>[2x]GMRNELPPENAYRILESGPIVLVSTRGADGRANLMTMGFH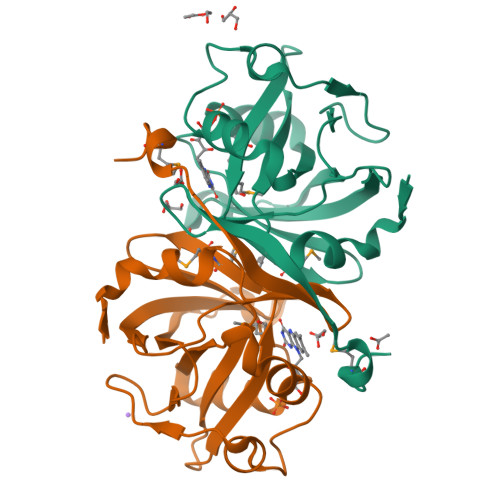MMMQHEPPLVGAIIGPWDYSHQALSETGECVLAVPTVDLAETVVDIGNCSGDALDKFGHFGLTPVPAQTVDAPLVRQCWANLECRVVDDGWARRYNLWVLEVQRIWIDTARKETRLIHHQGDGRFSVDGDTLDLGERMTKWRHLMG>MHHHHHHGSMSNEQTFIAIKPDGVQRGLIGPIISRFENRGFKLVAMKLVSPPQSQLEQHYADLSDKPFFKGLVSYMLSGPICAMVWEGRDVVKTGRTILG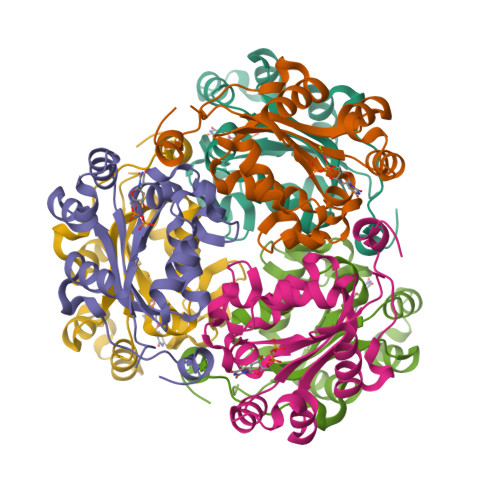ATNPLASAPGTIRGDFAIDVGRNVCHGSDSVENAKKEIALWFKPEELISWKSATFDWVYEKA[6x]1-(3-{[(2-aminoethyl)sulfanyl](diphenyl)methyl}phenyl)ethanone | C23 H23 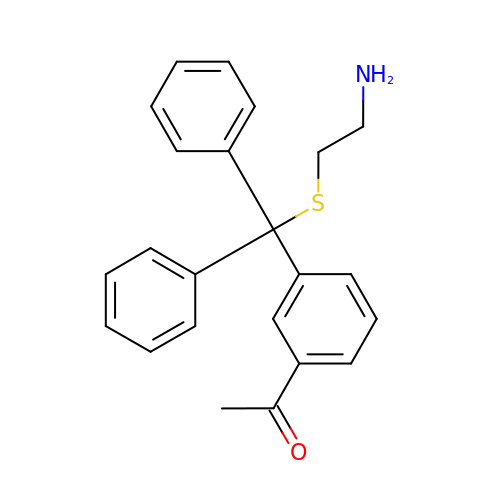N O S | FYVIRCUVQLOZOS-UHFFFAOYSA-N Yellow fever virus (YFV) is a re-emerging flavivirus that causes severe hepatic disease and mortality in humans. Crystallographic studies have resolved the structure of the YFV E protein and shown that its domain architecture is similar to related flaviviruses, with three N-terminal ectodomains, known as domains I (DI), II (DII) and III (DIII) and a stem anchor region known as the transmembrane domain (TM). Here we use a chimeric virus platform to resolve the first high resolution cryo-EM structures of YFV. Stark differences in particle morphology and homogeneity are observed between vaccine and virulent strains of YFV, and these are found to have significant implications on antibody recognition and neutralisation.

Introduction of R380 into bYFVES504 also resulted in more homogenous virions, allowing for its ASU to be resolved to a high resolution. The symmetry expanded local reconstruction method was used to resolve the ASU of bYFVES504 T380R to an initial resolution of 3.2 Å. To help elucidate all particle stabilising interactions that might be mediated by T380R, the symmetry expanded map was further refined after a focussed 3D classification around the previously ill-defined icosahedral three-fold axis. This resulted in two final maps with the three-fold axis E protein in two discrete states, which we designated up and down. While the global resolution of these maps are similar to the previous, the three-fold axis E protein is well resolved in the down map, allowing accurate modelling of the E protein in all three positions. Residue R380, which is located on a non-surface exposed loop of E-DIII, makes contacts with neighbouring E proteins at three unique inter-raft interfaces. The five-fold axis E protein R380 residue makes two intermolecular bonds with the backbone carbonyl groups of D382 and R384 and the two-fold axis E protein R380 residue forms a salt bridge with E87. In the down conformation, the three-fold axis E protein R380 residue makes a bond with the side chain hydroxyl of T133, while this contact is not observed in the up position. The atomic model of the bYFVES504 T380R ASU was then compared with the atomic model of the bYFVES504/DIII17D ASU and was found to be highly similar (rigid body whole ASU Cα RMSD: 0.82 Å). Instead, we propose that the three inter-raft interactions mediated by R380 act together to lock the smooth mature virion structure, and that this conformational stabilisation propagates down to the dimer level.

>[3x]AHCIGITDRDFIEGVHGGTWVSATLEQDKCVTVMAPDKPSLDISLETVAIDGPAEARKVCYSAVLTNVKINDKCPSTGEAHLEEENEGDNACKRTYSDRGWGNGCGLFGKGSIVACAKFTCAKSMSLFEVDQTKIQYVIRAQLHVGAKQENWNTDIKTLKFDALSGSQEAEFTGYGRATLECQVQTAVDFSNSYIAEMEKESWIVDKQWAQDLTLPWQSGSGGVWREMHHLVEFEPPHAATIKVLALGNQEGSLKTALTGAMRVTKDTNNSKLYKLHGGHVACRVKLSALTLKGTSYKMCTDKMSFVKNPTDTGHGTAVMQVKVPKGAPCRIPVMVADDLTAAVNKGILVTVNPIASTNDDEVLIEVNPPFGDSYIIVGRGDSRLTYQWHK> MRCIGISNRDFVEGVSGGSWVDIVLEHGSCVTTMAKNKPTLDFELIETEAKQPATLRKYCIEAKLTNTTTDSRCPTQGEPSLNEEQDKRFVCKHSMVDRGWGNGCGLFGKGGIVTCAMFTCKKNMKGKVVQPENLEYTIVITPHSGEEHAVGNDTGKHGKEIKITPQSSITEAELTGYGTVTMECSPRTGLDFNEMVLLQMENKAWLVHRQWFLDLPLPWLPGADTQGSNWIQKETLVTFKNPHAKKQDVVVLGSQEGAMHTALTGATEIQMSSGNLLFTGHLKCRLRMDKLQLKGMSYSMCTGKFKVVKEIAETQHGTIVIRVQYEGDGSPCKIPFEIMDLEKRHVLGRLITVNPIVTEKDSPVNIEAEPPFGDSYIIIGVEPGQLKLNWFKKGSSIGQMIETTMRGAKRMAILGDTAWDFGSLGGVFTSIGKALHQVFGAIYGAAFSGVSWIMKILIGVIITWIGMNSRSTSLSVS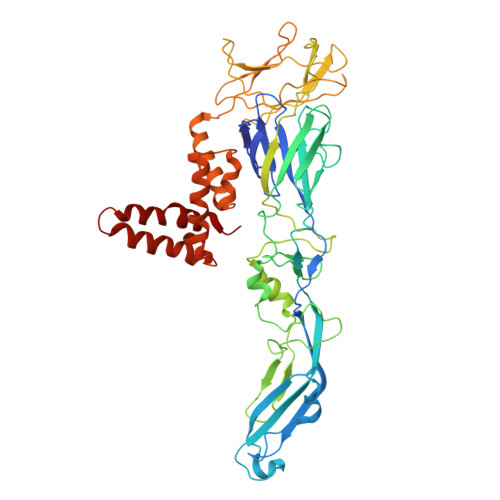LVLVGVVTLYLGVMVQA> SVDHGFLVTRHSQTTDDPQCPPGTKILYHGYSLLYVQGNERAHGQDLGTAGSCLRKFSTMPFLFCNINNV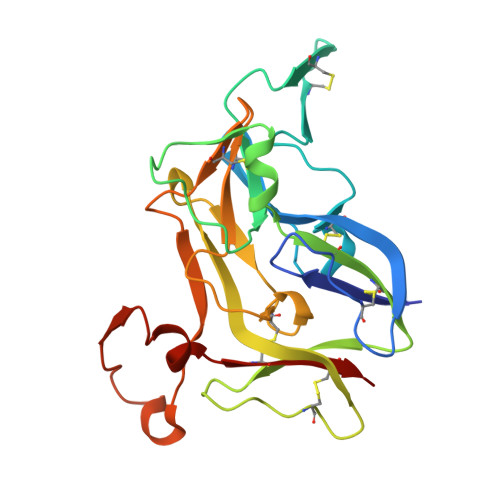CNFASRNDYSYWLSTPEPMPMSMAPITGENIRPFISRCAVCEAPAMVMAVHSQTIQIPQCPTGWSSLWIGYSFVMHTSAGAEGSGQALASPGSCLEEFRSAPFIECHGRGTCNYYANAYSFWLATIERSEMFKKPTPSTLKAGELRTHVSRCQVCMRRT L-GULURONIC ACID 6-PHOSPHATE 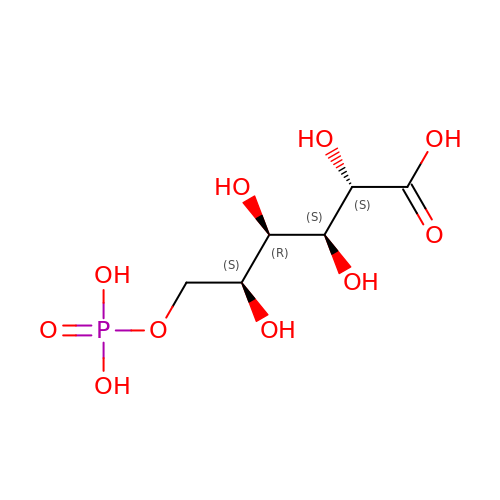| C6 H13 O10 P | BIRSGZKFKXLSJQ-QTBDOELSSA-N>SELQTEGRTRNHGHNVCSTWGNFHYKTFDGDVFRFPGLCDYNFASDCRGSYKEFAVHLKRGPGQAEAPAGVESILLTIKDDTIYLTRHLAVLNGAVVSTPHYSPGLLIEKSDAYTKVYSRAGLTLMWNREDALMLELDTKFRNHTCGLCGDYNGLQSYSEFLSDGVLFSPLEFGNMQKINQPDVVCEDPEEEVAPASCSEHRAECERLLTAEAFADCQDLVPLEPYLRACQQDRCRCPGGDTCVCSTVAEFSRQCSHAGGRPGNWRTATLCPKTCPGNLVYLESGSPCMDTCSHLEVSSLCEEHRMDGCFCPEGTVYDDIGDSGCVPVSQCHCRLHGHLYTPGQEITNDCEQCVCNAGRWVCKDLPCPGTCALEGGSHITTFDGKTYTFHGDCYYVLAKGDHNDSYALLGELAPCGSTDKQTCLKTVVLLADKKKNVVVFKSDGSVLLNELQVNLPHVTASFSVFRPSSYHIMVSMAIGVRLQVQLAPVMQLFVTLDQASQGQVQGLCGNFNGLEGDDFKTASGLVEATGAGFANTWKAQSSCHDKLDWLDDPCSLNIESANYAEHWCSLLKKTETPFGRCHSAVDPAEYYKRCKYDTCNCQNNEDCLCAALSSYARACTAKGVMLWGWREHVCNKDVGSCPNSQVFLYNLTTCQQTCRSLSEADSHCLEGFAPVDGCGCPDHTFLDEKGRCVPLAKCSCYHRGLYLEAGDVVVRQEERCVCRDGRLHCRQIRLIGQSCTAPKIHMDCSNLTALATSKPRALSCQTLAAGYYHTECVSGCVCPDGLMDDGRGGCVVEKECPCVHNNDLYSSGAKIKVDCNTCTCKRGRWVCTQAVCHGTCSIYGSGHYITFDGKYYDFDGHCSYVAVQDYCGQNSSLGSFSIITENVPCGTTGVTCSKAIKIFMGRTELKLEDKHRVVIQRDEGHHVAYTTREVGQYLVVESSTGIIVIWDKRTTVFIKLAPSYKGTVCGLCGNFDHRSNNDFTTRDHMVVSSELDFGNSWKEAPTCPDVSTNPEPCSLN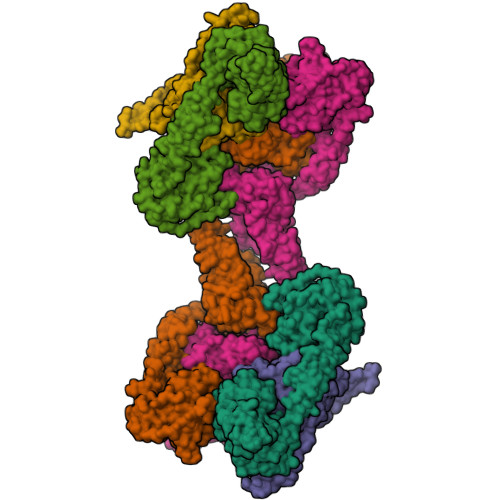PHRRSWAEKQCSILKSSVFSICHSKVDPKPFYEACVHDSCSCDTGGDCECFCSAVASYAQECTKEGACVFWRTPDLCPIFCDYYNPPHECEWHYEPCGNRSFETCRTINGIHSNISVSYLEGCYPRCPKDRPIYEEDLKKCVTADKCGCYVEDTHYPPGASVPTEETCKSCVCTNSSQVVCRPEEGKILNQTQDGAFCYWEICGPNGTVEKHFNICSITHHHHHH[6x]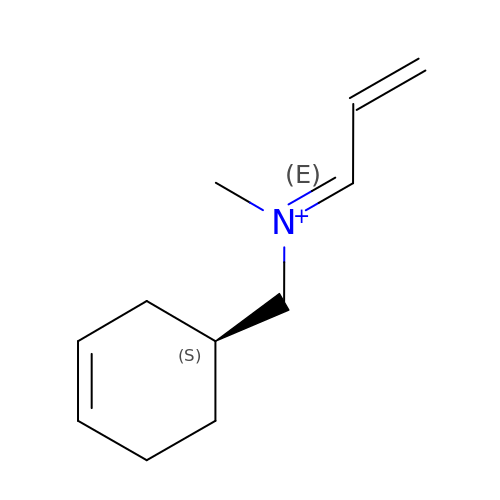N-[(E)-METHYL](PHENYL)-N-[(E)-2-PROPENYLIDENE]METHANAMINIUM | C11 H18 N | JBWDRSYKLIXPFB-LWMMSDEHSA-N>TWGVSSPKNVQGLSGSCLLIPCIFSYPADVPVSNGITAIWYYDYSGKRQVVIHSGDPKLVDKRFRGRAELMGNMDHKVCNLLLKDLKPEDSGTYNFR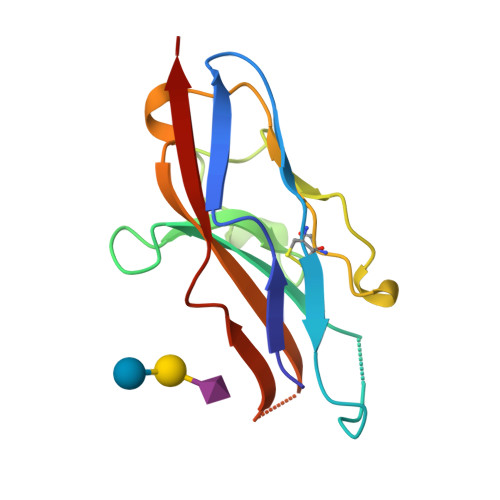FEISDSNRWLDVKGTTVTVTTD[3x]>ASAWPEEKNYHQPAILNSSALRQIAEGTSISEMWQNDLQPLLIERYPGSPGSYAARQHIMQRIQRLQADWVLEIDTFLSQTPYGYRSFSNIISTLNPTAKRHLVLACHYDSKYFSHWNNRVFVGATDSAVPCAMMLELARALDKKLLSLKTVSDSKPDLSLQLIFFDGEEAF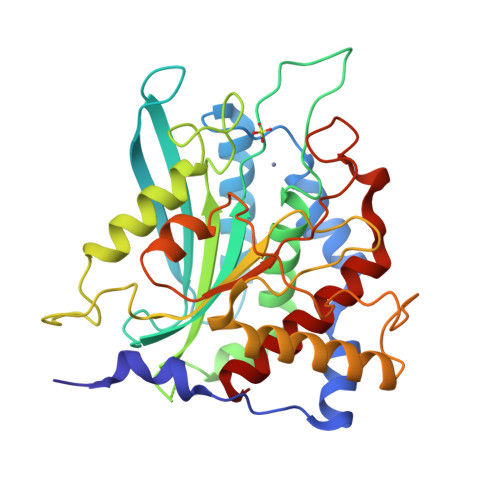LHWSPQDSLYGSRHLAAKMASTPHPPGARGTSQLHGMDLLVLLDLIGAPNPTFPNFFPNSARWFERLQAIEHELHELGLLKDHSLEGRYFQNYSYGGVIQDDHIPFLRRGVPVLHLIPSPFPEVWHTMDDNEENLDESTIDNLNKILQVFVLEYLHL[2x]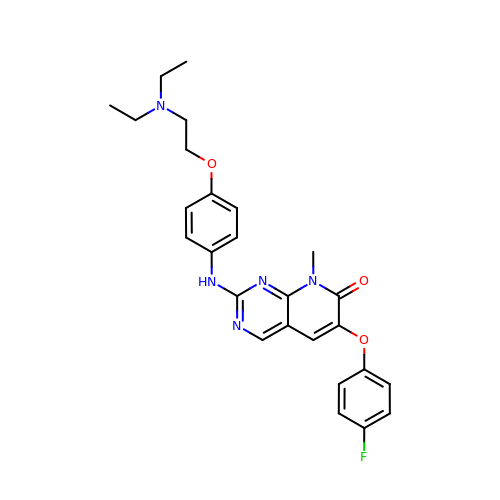2-({4-[2-(diethylamino)ethoxy]phenyl}amino)-6-(4-fluorophenoxy)-8-methylpyrido[2,3-d]pyrimidin-7(8H)-one | C26 H28 F N5 O3 | PAJOHXKWGHBVDS-UHFFFAOYSA-N> MEDKGKTFFGQPLGLSTLFMTEMWERFSYYGMRAILLYYMWFLISTGDLHITRATAASIMAIYASMVYLSGTIGGFVADRIIGARPAVFWGGVLIMLGHIVLALPFGASALFGSIILIIIGTGFLKPNVSTLVGTLYDEHDRRRDAGFSIFVFGINLGAFIAPLIVGAAQEAAGYHVAFSLAAIGMFIGLLVYYFGGKKTLDPHYLRPTDPLAPEEVKPLLVKVSLAVAGFIAIIVVMNLVGWNSLPAYINLLTIVAIAIPVFYFAWMISSVKVTSTEHLRVVSYIPLFIAAVLFWAIEEQGSVVLATFAAERVDSSWFPVSWFQSLNPLFIMLYTPFFAWLWTAWKKNQPSSPTKFAVGLMFAGLSFLLMAIPGALYGTSGKVSPLWLVGSWALVILGEMLISPVGLSVTTKLAPKAFNSQMMSMWFLSSSVGSALNAQLVTLYNAKSEVAYFSYFGLGSVVLGIVLVFLSKRIQGLMQGVEGSENLYFQ

To address this question, we determined high-resolution crystal structures of a bacterial homologue to the mammalian PepT1 protein from Streptococcus thermophilus, PepTSt in complex with physiologically relevant di- and tripeptides in addition to a peptide-free apo form. The POT/PTR family contains a number of conserved sequence motifs and a conserved architecture consisting of 12 or 14 transmembrane α-helices arranged into N (H1–6)- and C-terminal (H7–12) bundles 3,10–12. A centrally located peptide-binding site is highly conserved between prokaryote and eukaryote members, with both operating via similar transport mechanisms. Conserved pairs of salt bridge interactions coordinate structural rearrangements that lead to the vectorial co-transport of peptides and protons across the membrane 3,11.

Comparing the structures of PepTSt in the peptide-bound states with a high-resolution peptide-free apo state determined to 2.35 Å reveals that the Ala-Phe complex assumes a more compact structure. The movement appears localized to the C-terminal bundle and occurs following intra-helical bending at residues Ser431 (H11), Asn328 (H8) and to a lesser extent at Asn156 (H5), the latter two side chains making direct H-bond interactions with the Ala-Phe peptide. The cytoplasmic ends of H10 and H11 form an intracellular gate with a hinge region located around Gly407 (H10) and Trp427 (H11) 3. C Zoomed in view of H11 showing the formation of the hydrophobic pocket around the phenylalanine side chain of the Ala-Phe peptide (coloured helices) and the dissolution of the pocket upon adopting the more open structure observed in the Apo structure (grey). The structure of the Ala-Phe complex suggests that the closing of this gate around the dipeptide results in the formation of the hydrophobic pocket, which forms to accommodate the bulky phenyl side chain of the ligand. These observations are consistent with an induced fit mechanism within the POT/PTR family with peptide binding facilitating structural rearrangement of the TM helices at sites of interaction with the peptide ligand.>ASNFTQFVLVDNGGTGDVTVAPSNFANGV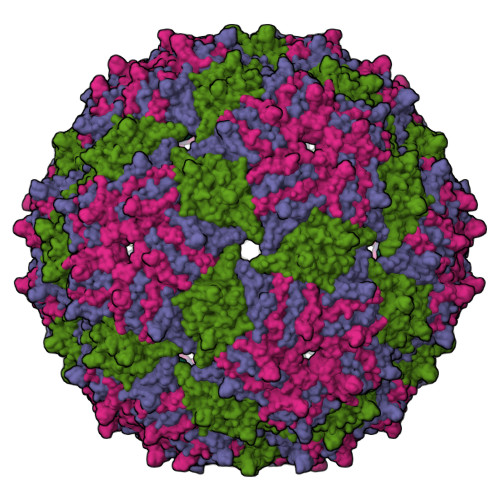AEWISSNSRSQAYKVTCSVRQSSAQNRKYTIKVEVPKVATQTVGGVELPVAAWRSYLSMKLTIPIFATNSDCELIVKAMQGLLKDGNPIPSAIAANSGIY[3x]>[4x]SDILGMLKSLHQLQVE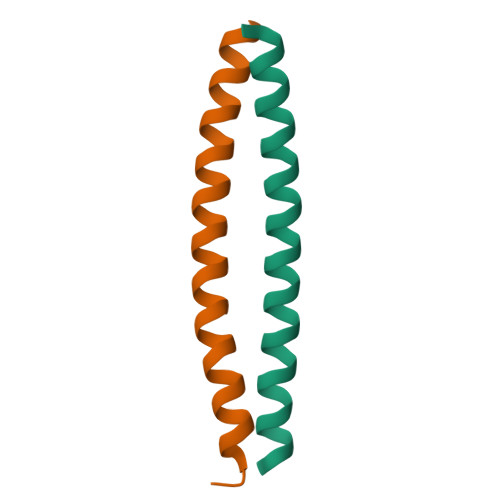NRRLEEQIKNLTAKKERLQLLNAQLSV;>[4x]SQIEWAKARVEKLRKRNQALKSQTSELQRQIAELEASNAELKK>MIDLNIMKVANYINGEFKEPSTGAFQVKTSPVDGSKIAEVPRSGREDAREAIDSAFEALKAWANIPAIRRAEYLYKMLEVFRQMKEDFMKILTVEGGGTYRKVWGEVVFTERLIQNAAELARHYQGRVLQSDSESTISVVFKRSKGVVGVITPWNYPLSISMKKIAHTLAVGNTVVYKPASDTPVTGWLIAQMVAKAGLPKGVFNLVIGPGPVVGEEIVTHKRVAHVTFTGESSTGREIAAKAAGTLKTVTLELGGSDPLIILDDVDVDYAARLAVFASLFHQGQICTSAKRIIVHKAVADKFIERYVHYVKMLRIDDPRKDEKVDLGPLINERQVALMKEFVDDAVSRGGRLLIGGRSWGNFF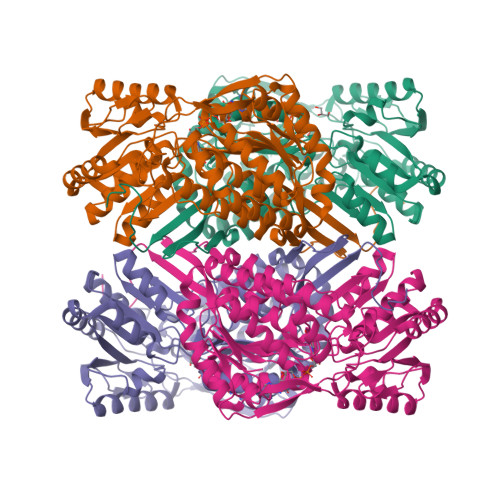EPAIFVDVDRNFRIMREEVFGPVRPIVVVENDDQAVEVANDTDYGLSGAVLTNNVNRAFRIAEAVESGMFHINDVTFLEESHVPFGGIKASGVGREGGEWSFHETTYDRWVTVTLRTRRFPIPSALK[8x]> AQSVPWGISRVQAPAAHNRGLTGSGVKVAVLDTGISTHPDLNIRGGASFVPGEPSTQDGNGHGTHVAGTIAALDNSIGVLGVAPSAELYAVKVLGASGSGAISSIAQGLEWAGNNGMHVANLSLG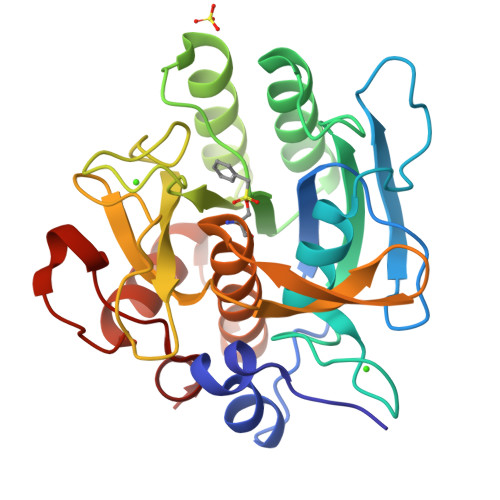SPSPSATLEQAVNSATSRGVLVVAASGNEGAGSIDYPARYANAMAVGATDQNNNRASFSQYGAGLDIVAPGVNVQSTYPGSTYASLNGTSMATPHVAGAAALVKQKNPSWSNVQIRNHLKNTATSLGSTNLYGSGLVNAEAATR> KGSVVIVGR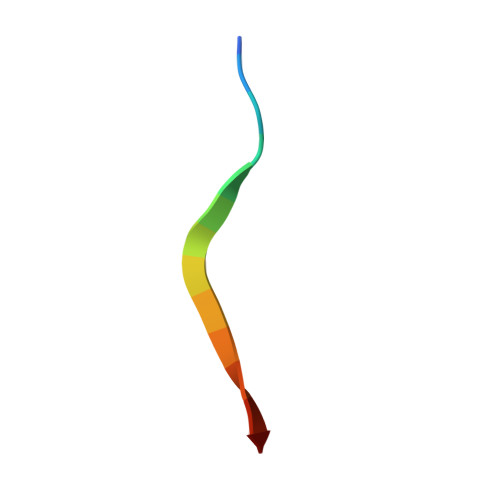IILSK>MNKVEPQESNAIRMIKEACEKNRRMMTDEAFRKEVEKRLYAGPSPELLAKLRVLWAANKEQ[4x];>MVKLSSDINLRDFGNNEYLSSVQDEAIRFATEQTDEILSLYSQHADTEGGRYVCADTFKELFPAFENKEDRATVNNAIHNSAAVLSSTQFDEVLKRDEPQKKEVIFVTGIPGSGKTSTVKNMMMQDTTKLLFEGQLARPQSAFRKIEQCLERNLEVTIVAVSMRAERASDNTYKRFNEYGRGASIGIMADIQANLPDGLKQIRDKFGDAVKIVGINQDRNSEFIDKFDDVIKMLSLGSQEQILGRLAEKIQSDFDSGKISRECFNQAKGSMDLESVFAKKEYSQQRVVTNSKGVTLETKSANELWSKVEQIPVTG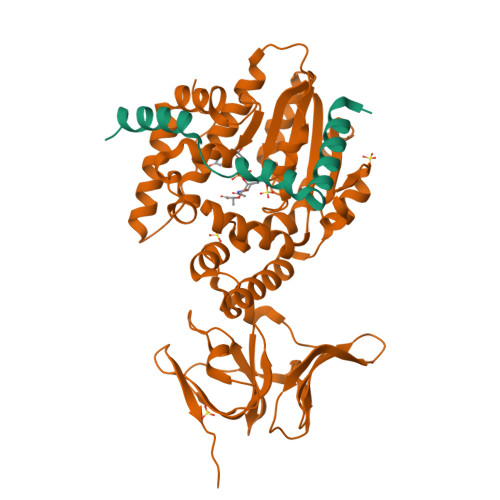MKAGIYLLGQAKKAETGQTYSGEIIYKDAAAVFQKTKNGLVRHNATHNEERLAKLVEIGQNVSIGSNKGKLIVKSLEYSAKKSISR[4x]>TEQTLFEQLNSKNVNDHTEQKNGLTYLAWSYAHQELKKIDPNYTVKVHEFPHPDINTENYFVPYLATPEGYFVQVSVTVKDSTETEWLPVLDFRNKSLAKGSATTFDINKAQKRCFVKASALHGLGLYIYNGEELPSASDNDITELEERINQFVNLSQEKGRDATIDKTMRWLKISNINKLSQKQIAEAHQKLDAGLKQLDSEEKQ[34x];>MGIRNRLSELLSERGLKISRVAKDVKIARSSLTSMAQNDSEMIRYDA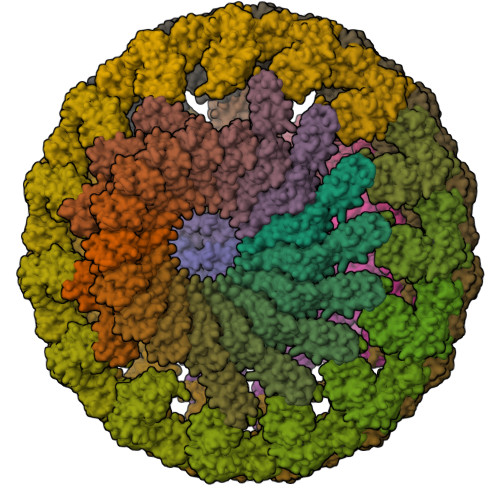IDKLCSYLHISPSEFFEHNPINFDFTFDEEPNYKINDVFEGFEVTANITHAFSIENFDFEILVDVELDNRQKLNFDLDVSYKETEKITNSQHRFIFTIKNEDENIGLKKYVDSLSAGLKNLLFKKINQKLSGYVSEIIVKNIDDIEELFPNKGEKSTTLHKEILQTDSRLSSDIFKEYGSHHHHHH[30x]>[2x]GFKQDIATLRGDLRTYAQDIFLAFLNKYPDERRYFKNYVGKSDQELKSMAK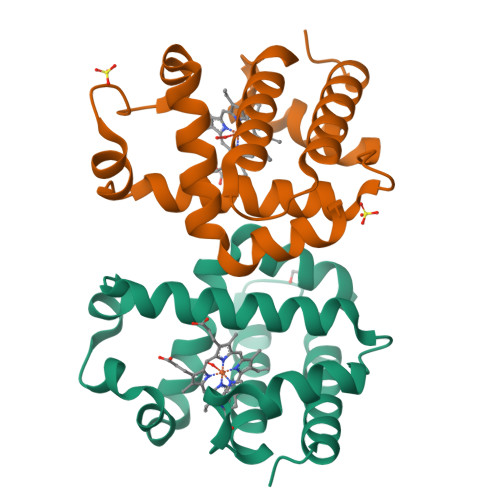FGDHTEKVFNLMMEVADRATDCVPLASDANTLVQMKQHSSLTTGNFEKLFVALVEYMRASGQSFDSQSWDRFGKNLVSALSSAGMK> MDLKVEIETLYEVSKILSSSLNLETTVPYIFRLLKKLMGFERLTLTIYD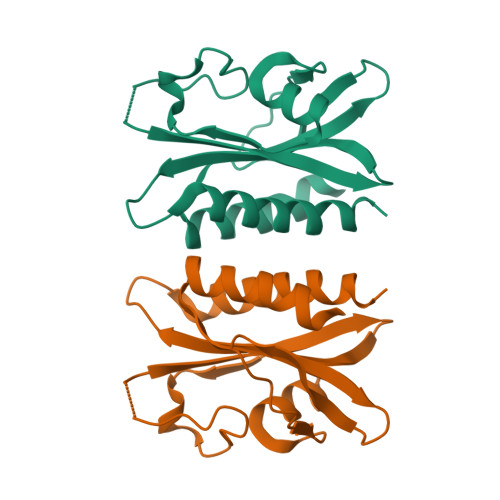PSTDQIVVRATSSGKFPKEGFKKGEGITGKVWKHGVPIVIPDISQEPEFLNKVWKRKKSKKKIAFIAVPIKSGGKVIGVLSADKEINEKDSLDEYTRFLSMIATLIANSFSLERKVQAERKS>[4x]ASGSPTGGQIVAGSGSIQTPSGNQMNIHQNSQNMVANWNSFDIGKGNTVQFDQPSSSAVALNRVVGGGESQIMGNLKANGQVFLVNPNGVLFGEGASVSTSGFVASTRDIKNDDFMNRRYTFSGGQKAGAAIVNQGELTTNAGGYIVLAADRVSNSGTIRTPGGKTVLAASERITLQLDNGGLMSVQVTGDVVNALVENRGLVSARDGQVYLTALGRGMLMNTVLNVSGVVEASGMHRQDGNIVLDGGDSGVVHLSGTLQADNASGQGGKVVVQGKNILLDKGSNITATGGQGGGEVYVGGGWQGKDSNIRNADKVVMQGGARIDVSATQQGNGGTAVLWSDSYTNFHGQIGAKGGETGGNGGRVETSSHGNLQAFGTVSASAA

One such adhesin, EtpA, is a 177 kDa or 1767 residues, secreted protein that bridges the tips of ETEC flagella to host epithelial glycans including human A blood group to promote bacterial adhesion, intestinal colonization and toxin delivery. EtpA is exported through a Gram-negative, two-partner secretion system (TPSS, type Vb) comprised of the secreted EtpA passenger (TpsA) protein and EtpB (TpsB) transporter that is integrated into the outer bacterial membrane. TpsA proteins share a conserved, N-terminal TPS domain followed by an extensive C-terminal domain with divergent sequence repeats. Outer membrane TspB proteins recognise the N-terminal TPS domain of their cognate TpsA to initiate exoprotein translocation across the outer membrane with simultaneous folding nucleated by the N-terminus.

The crystal structure of EtpA67-447 solved at 1.76 Å resolution revealed a right-handed parallel β-helix with two extra-helical hairpins and an N-terminal β-strand cap. The asymmetric unit of the EtpA67-447 crystals contained four symmetrically independent but equivalent monomers. Each monomer forms a triangular, right-handed β-helix of 13 turns (or rungs), where each turn consists of two or, more commonly, three roughly coplanar β-strands. Strands from adjacent turns align to create the parallel β-sheets PB1, PB2 and PB3 with 13, 11 and 14 β-strands, respectively. While β-strands β1 and β2 (red) form part of PB1 and PB2, they align antiparallel to the otherwise parallel β-sheets and serve to cap the β-helix. The loop connecting β-strands β9 and β10 is a type 1 β-turn and harbours a conserved NPNG motif critical for TpsA protein folding. The interior of the β-helix is dominated by hydrophobic, aliphatic residues, especially valine. Two loops connecting physically adjoining β-strands β12-β14 and β19-β22, are extended to create an extra helical domain consisting of α-helix α1 and β-strands β13, and β20 and β21, respectively. The extra-β-helical secondary structure elements all pack onto the outer face of β-sheet PB1 broadly alligned (anti-) parallel to its β-strands. Despite low sequence identities of EtpA67-447 with the other TPS domains (34% for HMW1-PP, 35% for HxuA, 27% for FHA30, and 23% for HpmA265), the domains all form analogous right-handed β-helices with tightly packed, hydrophobic cores and characteristic aromatic clusters in the first helical turn (W34, F47, F79, F88 and F99 in EtpA).Bacteriophage exclusion (‘BREX’) systems are multi-protein complexes encoded by a variety of bacteria and archaea that restrict phage by an unknown mechanism. The final gene in most type 1 BREX systems, termed ‘BrxL’, encodes a large protein (670–700 residues in various species), with much of its sequence predicted to adopt a fold corresponding to the chambered ATP-dependent AAA+ protein family, which are involved in a wide variety of cellular functions throughout all biological kingdoms. In this study we have demonstrated that the BrxL phage restriction factor is a multimeric DNA binding protein that displays ATP-dependent assembly on double stranded DNA.

EM grids of wild-type BrxL contained a mixture of particle sizes, with the majority appearing to comprise barrel-shaped multimers displaying seven-fold (heptameric) symmetry. The final CryoEM maps for the full size wild-type BrxL complex extended to approximately 3.5 Å resolution. The structure of the full-length BrxL assemblage was built and refined into that density using homology models of the NTD and AAA+ ATPase domains generated using AlphaFold combined with the crystal structure of the C-terminal domain described above. Ultimately the maps supported modeling 14 independently placed BrxL subunits arranged into a dimer of heptameric rings. In the resulting structure, each heptameric ring assembles via contacts between the NTD and central ATPase domains of adjacent monomers. Two such heptamers further associate with one another via tail-to-tail contacts between their CTDs. A large internal void in the interior of the protein chamber contains no significant electron density. The buried surface area between adjacent protein subunits around each heptameric ring (as calculated using the PISA webserver) is approximately 1100 Å2 and involves up to six directional side chain hydrogen bonds and salt bridges distributed between eleven residues within each interface. The buried surface area between each pair of CTDs around the equator of the assemblage (producing the tail-to-tail dimerization of two heptameric rings) is smaller (∼600 Å2). The structural rearrangements observed when comparing unbound, DNA-free heptameric BrxLWT assemblages to DNA-bound BrxLE280Q hexameric assemblages involve (1) a hinged motion centered around a peptide linker (residues 469 to 497) connecting the AAA+ ATPase domain and the CTD, and (2) a pivot of the two CTD domains, relative to one another, in each ‘tail-to-tail’ subunit interface around the BrxL equator.

>MESANDKELDQLLNEHFAGRVVRKDLTKLIKEGANVPVYVLEYLLGMYCASDDPEIIEQGLRNVKTVLAENYVRPDEAEKVKSLVRERGSYKVIDRVTVKLNERKDKYEASFSNLGIKDAEISAGIVKEYEKLLVGGIWVIATLSYYFEEGQTSSPFGVSLLKPIQMPNMNMDELFSGRAALSTDQWRESLIRSIGMEPASLKEDVQWHLLARMVPFVENNYNVCELGPRGTGKSHIYKECSPNSILVSGGQTTVANLFYNMSSRRIGLVGLWDVVAFDEVAGISFKDKDGVQIMKDYMASGSFARGREQMEASASMVFVGNINQSVESLVKTSHLLAPFPEAMIDSAFFDRFHAYIPGWEIPKMRPEFFTNRYGLIVDYLAEFFREMRKRSFADSIEKYFKLGNNLNQRDVIAVRKTVSGLMKLLYPHGQFNKEDVRQCLEYALQVRRRVKEQLKKIGGMEFYDVHFSYIDNDTLEEHFVSVKEQGGGGLIPEGPAKPGFLYTIGLSNKGMPGLYRLELQVTKGSGKLATSGLWNSSSAKEQVKIAFDYFKANASRISGGSKVMEHDFHLHVVELQNTGPLSHLALPSLVAFASGLLGRSVQSQMVVLGDMSLGGSVTPVESIAECLQVAFDAGAKKVALPMSSAADIPTIPVELFTKFQTSFYADPVDAVFKGLGVD[14x]> KMLEGQNA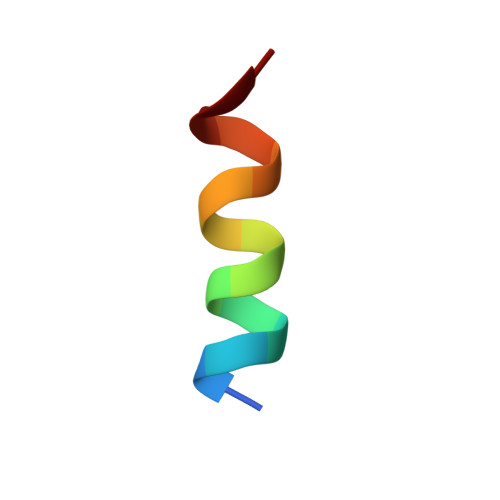HFRYKNR> SLNTDLGLGHNGVRISLNYFDGLPDPSLLNSLYSNELKLIFKSLLKRDETTKEKALMDLSNLISDFNQNEYFFNDIFLLCWSQIYAKLIISDYKVIRLQSHQITIMLVKSLRKKISKFLKDFIPLILLGTCELDYSVSKPSLNELTECFNK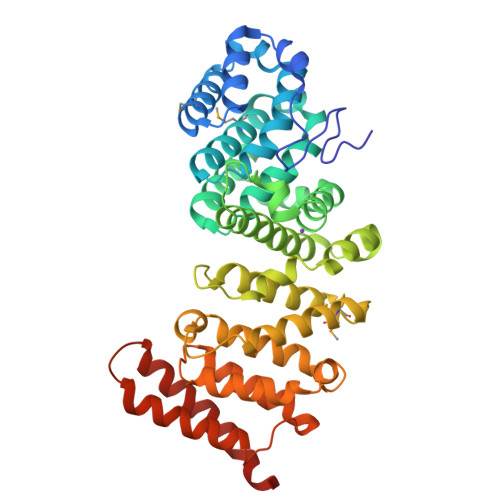DPAKINALWAVFQEQLLNLVKEIVVNENEDTISDERYSSKEESEFRYHRVIASAVLLLIKLFVHNKDVSERNSSSLKVILSDESIWKLLNLKNGQNTNAYETVLRLIDVLYTRGYMPSHKNIMKLAVKKLLKSLTHITSKNILKVCPVLPSILNLLATLDDYEDGTIWSYDKSSKEKVLKFLSVSRTSPSPGFFNAVFALYSSTKRHSFLDYYLEWLPFWQKSVQRLNEKGFSARNSAEVLNEFWTNFLKFAEDSSEERVKKM>GPLGSPEFQKTKPFSVPNLPLNTLSNSRVPSLIRSMMVSRDHGQMVQFQNGRVTLDGQLQGTTPTSASQLCKIRGSVFHANG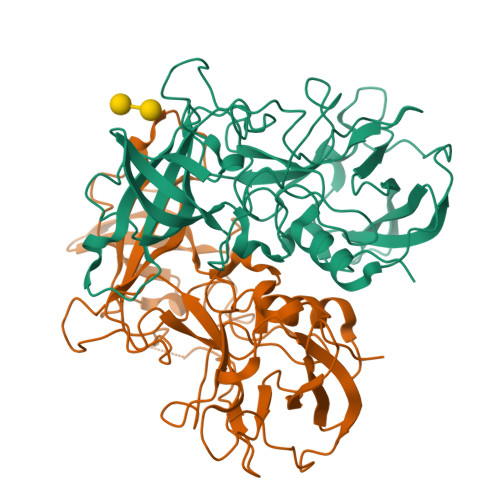GNGYNLTELDGSPYHAFESPAPIGFPDLGECDWHMEASPTTQFDTGDVIKQINVKQEAAFAPHLGTIQADGLSDVSVNTNMIAKLGWVSPASDGHRGNVDPWVIPRYGSTLTEAAQLAPPIYPPGFGEAIVFFMSDFPIAHGANGLSVPCTIPQEFVTHFVNEQAPTRGEAALLHYLDPDTHRNLGEFKLYPEGFMTCVPNSSGTGPQTLPINGVFVFVSWVSRFYQLKPVGTAGPARSLGIRRS[4x]>[4x]KRKIIFLSSPYGFSQQQKTLLLPPIVRALEALGIEVWEPFARNNQIDFSQADWAYRVAQADLQDVKNCDGIFAVVNGTPPDEGVMVELGMA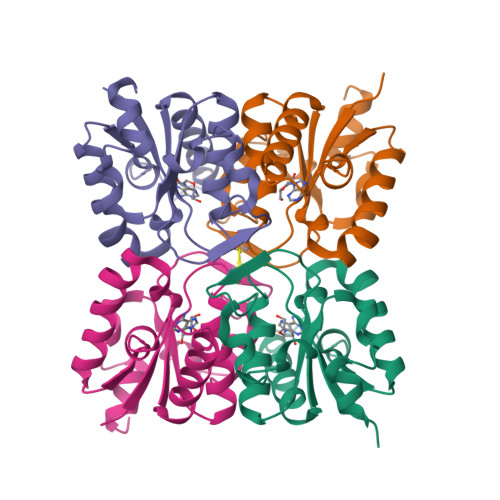IALNKAIFLFRDDFRRCSDNERYPLNLMLFAGLPEIGWENYYYTSVDEIQSHDKALYKWLTGM>[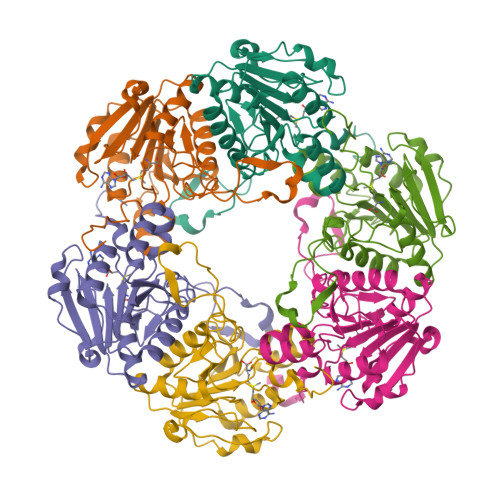6x]MNDYSRQNFQDLNLFRGLGEDPAYHPPVLTDRPRDWPLDRWAEAPRDLGYSDFSPYQWRGLRMLKDPDTQAVYHDMLWELRPRTIVELGVYNGGSLAWFRDLTKIMGIDCQVIGIDRDLSRCQIPASDMENITLHQGDCSDLTTFEHLREMAHPLIFIDNAHANTFNIMKWAVDHLLEEGDYFIIEDMIPYWYRYAPQLFSEYLGAFRDVLSMDMLYANASSQLDRGVLRRVAAKQ>ATTVQGFDISNHQKSVNFEAAKKDGAQFVMIKATEGTTYKDTVFNSHYTGATKAGLLRGGYHFARPDKSTGSTQAKFFLKNGGGWSDDNRTLPGMLDIEYNPYGATCYGLSHSQMVAWIHDFVNEYHHATSRWPMIYTTADWWN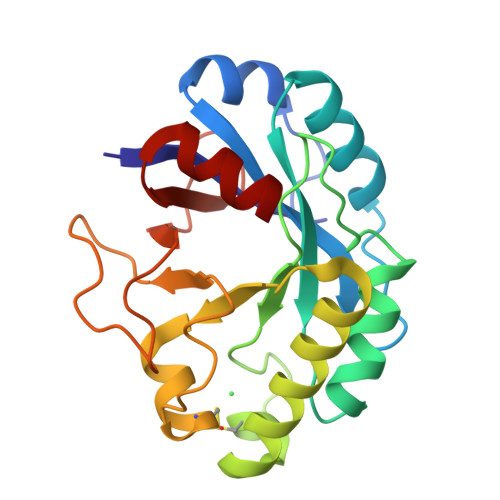RCTGNAKGFGDKCPLVLAAYSSSPPKTIPGDWKTWTIWQNSDKYKHGGDSDKFNGPMTQLRKLASG[6x]> GRQFGHLTRVRHLITYSLSPFEQRPFPHYFSKGVPNVWRRLRACIL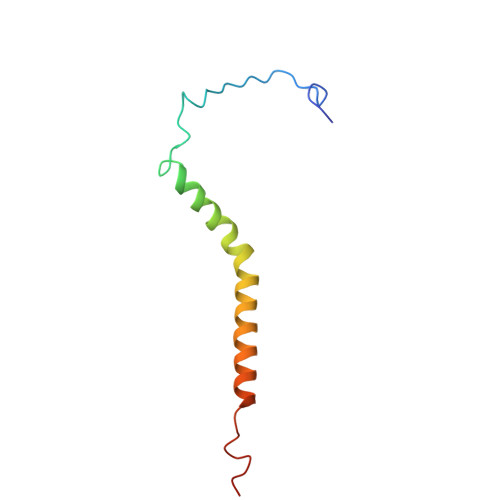RVAPPFLAFYLLYTWGTQEFEKSKRKNPAAYVNDR>TADELVFFVNGKKVVEKNADPETTLLAYLRRKLGLRGTKLGCGEGGCGACTVMLSKYDRLQDKIIHFSANACLAPICTLHHVAVTTVEGIGSTKTRLHPVQERIAKSHGSQCGFCTPGIVMSMYTLLRNQPEPTVEEIEDAFQGNLCRCTGYRPILQGFRTFAK[2x];>[2x]PKQLRFEGERVTWIQASTLKELLDLKAQHPEAKLVVGNTEIGIEMKFKNQLFPMIICPAWIPELNAVEHGPEGISFGAACALSSVEKTLLEAVAKLPTQKTEVFRGVLEQLRWFAGKQVKSVASLGGNIITASPISDLNPVFMASGTKLTIVSRGTRRTVPMDHTFFPSYRKTLLGPEEILLSIEIPYSREDEFFSAFKQASRREDDIAKVTCGMRVLFQPGSMQVKELALCYGGMADRTISALKTTQKQLSKFWNEKLLQDVCAGLAEELSLSPDAPGGMIEFRRTLTLSFFFKFYLTVLKKLG;>DTVGRPLPHLAAAMQASGEAVYCDDIPRYENELFLRLVTSTRAHAKIKSIDVSEAQKVPGFVCFLSADDIPGSNETGLFNDETVFAKDTVTCVGHIIGAVVADTPEHAERAAHVVKVTYEDLPAIITIEDAIKNNS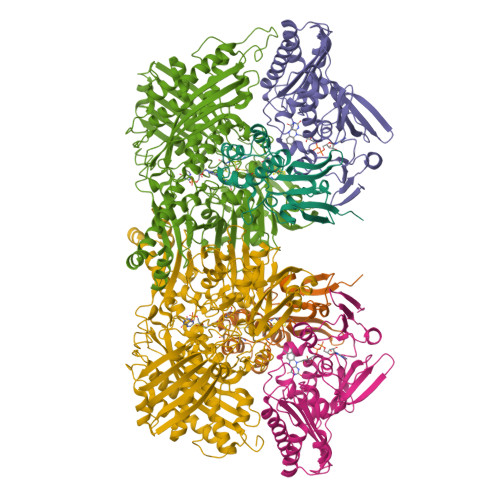FYGSELKIEKGDLKKGFSEADNVVSGELYIGGQDHFYLETHCTIAIPKGEEGEMELFVSTQNAMKTQSFVAKMLGVPVNRILVRVKRMGGGFGGKETRSTLVSVAVALAAYKTGHPVRCMLDRNEDMLITGGRHPFLARYKVGFMKTGTIVALEVDHYSNAGNSRDLSHSIMERALFHMDNCYKIPNIRGTGRLCKTNLSSNTAFRGFGGPQALFIAENWMSEVAVTCGLPAEEVRWKNMYKEGDLTHFNQRLEGFSVPRCWDECLKSSQYYARKSEVDKFNKENCWKKRGLCIIPTKFGISFTVPFLNQAGALIHVYTDGSVLVSHGGTEMGQGLHTKMVQVASKALKIPISKIYISETSTNTVPNSSPTAASVSTDIYGQAVYEACQTILKRLEPFKKKNPDGSWEDWVMAAYQDRVSLSTTGFYRTPNLGYSFETNSGNAFHYFTYGVACSEVEIDCLTGDHKNLRTDIVMDVGSSLNPAIDIGQVEGAFVQGLGLFTLEELHYSPEGSLHTRGPSTYKIPAFGSIPTEFRVSLLRDCPNKKAIYASKAVGEPPLFLGASVFFAIKDAIRAARAQHTNNNTKELFRLDSPATPEKIRNACVDKFTTLCVTGAPGNC[2x]> EWEA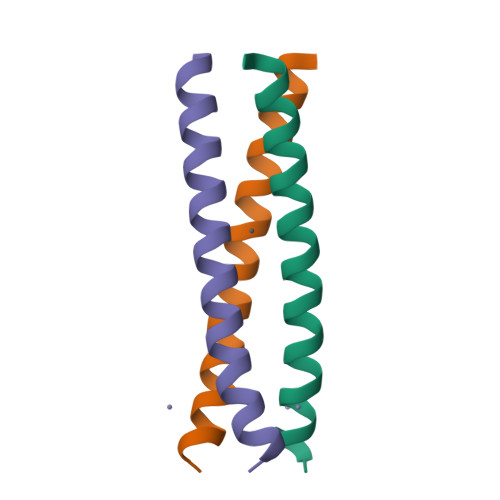LEKKLAAAESKCQALEKKLQALEKKLEALEHG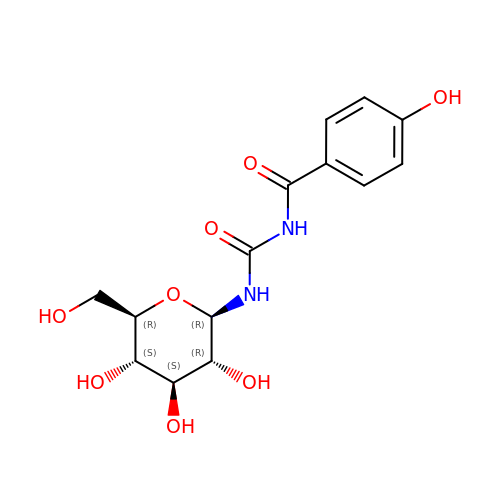N-{[(4-hydroxyphenyl)carbonyl]carbamoyl}-beta-D-glucopyranosylamine | C14 H18 N2 O8 | YHOJJLBUFKEFNL-BZNQNGANSA-N> MADEEDPWGFDDGGEEEKAASTQAGTPAPPSKAPSVASDHKADSVVAGTPANEEAAPEEVEEIKAPPPPPEDDGYRKPVQLYRHWVRPKFLQYKYMYNYRTNYYDDVIDYIDKKQTGVAREIPRPQTWAERVLRTRNISGSDIDSYAPAKRDKQLIQTLAASIRTYNYHTKAYINQRYASVL

Striated muscle thick filaments are composed of myosin II and several non-myosin proteins which define the filament length and modify its function. Myosin II has a globular N-terminal motor domain comprising its catalytic and actin-binding activities and a long α-helical, coiled tail that forms the dense filament backbone. Here we report an improved structure at 4.7 Å resolution of flight muscle thick filaments from a wild type strain of Drosophila melanogaster. Improved resolution for the non-myosin proteins resolves the entire length of flightin within the annulus of myosin tails, resolves the ambiguity for one unassigned density, and improves the shape of the stretchin-klp densities on the surface of the filament backbone.

Studies of the flightin amino acid sequences from many species identified a highly conserved domain in the middle of the sequence, residues W85-R131 in Drosophila, dubbed the “WYR” domain due to its enrichment in tryptophan, tyrosine, and arginine. Application of the structure prediction program AlphaFold to the Drosophila flightin sequence produced a structure for the WYR domain that was an excellent fit to the central density. The WYR domain-predicted structure consists of a pair of α-helices connected by a loop. The orientation of the predicted WYR domain structure identifies the V-shaped density as coming from the sequence on its N-terminal side and the inner extended density as coming from the C-terminal side of the flightin sequence. To obtain the final model, we removed the N-terminal residues P69-K95 from the AlphaFold model and rebuilt them de novo in COOT. In addition, the residues G140-L182 were also rebuilt de novo to fit the density. The atomic model begins at residue P69 leaving 68 N-terminal residues disordered. The myosin mutation E1554K prevents incorporation of flightin into Drosophila flight muscle thick filaments. The Drosophila flightin atomic model places flightin residue R87 in position to form a salt bridge with E1554. The second region of interaction contains a salt bridge between myosin residue E1557 with flightin loop-1 residue R124.>[2x]MYGKGKSNSSAVPSDSQAREKLALYVYEYLLHVGAQKSAQTFLSEIRWEKNITLGEPPGFLHSWWCVFWDLYCAAPERRETCEHSSEAKAFHDY;> YTEFAPPPTPMVDHLVASNPFEDDFGA;> GIGRHTPYGNQTDYRIFELNKRLQNWTEECDNLWWDAFTTEFFEDDAMLTITFCLEDGPKRYTIGRTLIPRYFRSIFEGGATELYYVLKHPKEAFHSNFVSLDCDQGSMVTQHGKPMFTQVCVEGRLYLEFMFDDMMRIKTWHFSIRQHRELIPRSILAMHAQDPQMLDQLSKNITRCGLSNSTLNYLRLCVILEPMQELMSRHKTYSLSPRDCLKTCLFQKWQRMVAPP

The Wnt enhanceosome is responsible for transactivation of Wnt-responsive genes and a promising therapeutic target for treatment of numerous cancers with Adenomatous Polyposis Coli (APC) or β-catenin mutations. Here we show that B-cell lymphoma 9 protein (BCL9), Pygopus (Pygo), LIM domain-binding protein 1 (LDB1) and single-stranded DNA-binding protein (SSBP) form a stable core complex within the Wnt enhanceosome. Their mutual interactions rely on a highly conserved N-terminal asparagine proline phenylalanine (NPF) motif of Pygo, through which the BCL9-Pygo complex binds to the LDB-SSBP core complex. Pygo proteins contain three highly conserved domains: a nuclear localization signal (NLS), an N-terminal homology domain (also called N-box) including a highly conserved NPF motif and a C-terminal plant homology domain (PHD).

To provide a structural basis for the Pygo2-ChiLS interaction, we determined the crystal structure of the ternary complex assembled from human Pygo2(58–84), LDB1(56–285) and SSBP2(1–94) at 2.45 Å resolution. In our crystal lattice, there is one Pygo2 molecule and one LDB1-(SSBP2)2 complex in each asymmetric unit. Pygo2(58–84) adopts an unstructured loop, confirming secondary structure predictions. Its N-terminus is located on the surface of the SSBP2 dimer whereas its C-terminus protrudes into a pocket formed by the interface between LDB1 and SSBP2. The structure of the ChiLS core complex is almost identical to the previously reported structure of ChiLS30 (RMSD = 0.366 Å), indicating that the binding of Pygo2 to ChiLS does not alter its overall conformation. However, there was one marked conformational difference for a loop of SSBP2 (amino acids 49–51): a lysine residue within this loop (K50) shifted by about 6.6 Å, tilting away from the bound Pygo2, thereby avoiding a clash with Pygo2 M68 and L72. Pygo2(58–84) interacts with ChiLS through three sets of contacts. Firstly, F68, W69 and Y72 of one SSBP2 molecule and Y25, F60 and W64 of another, together with L245 and I248 of LDB1, form a deep hydrophobic pocket that interacts with NPF (residues 76–78) of Pygo2(58–84). Secondly, the PPP cluster (residues 63–65) and L72 of Pygo2(58–84) are accommodated by a hydrophobic groove formed largely by W48 and H62 of SSBP2. Thirdly, LDB1 R232 and R244 undergo tight hydrogen bonds with D80 within the NPF motif of Pygo2, and we also note salt bridges between Pygo2 E79 and LDB1 N237 and N241.> GPLGSEKIEKDNAFAFDLLQTTRKHVTEANVFISPLSVSMALNMTLNGAAGVTADEMKTALRETGYTMEDINEYSHSLREALLKVDPSTTIGMANSIWYKQGELVKEPFILANRTHYDAEVK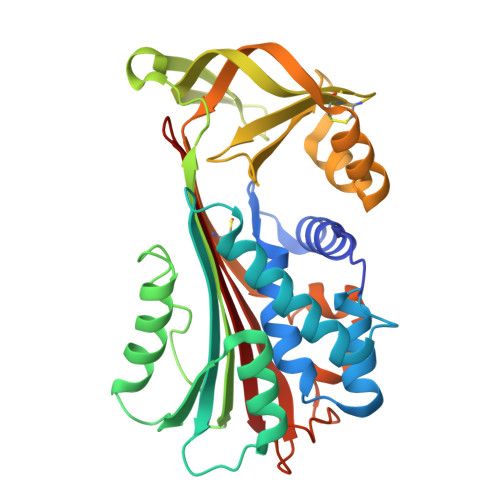AVDFSSPATLPAINGWCAQKTNDKITKILDYIPGNAFMYLINAVYFKGIWVTQFKKSDTKRAPFRKADGTTQEVNMMAQKSTFGYTTDECCQYLEMDYGNKAFSMIVMLPNEGQTTRDVIEQLDNKHWSMIIKGIRPTQVSLRMPRFKTECKYGLEKKILPEMGMNVPFTETADFPGITDAAIFISRVIHKTFVQVDEEGTEAAAVTAVEMVKT>MYSKIKISGTIEVVTGLHIGGGGESSMIGAIDSPVVRDLQTKLPIIPGSSIKGKMRNLLAKHFGLKMKQESHNQDDERVLRLFGSSEKGNIQRARLQISDAFFSEKTKEHFAQNDIAYTETKFENTINRLTAVANPRQIERVTRGSEFDFVFIYNVDEESQVEDDFENIEKAIHLLENDYLGGGGTRGNGRIQFKDTNIETVVGEYDSTNLKIK[4x];> MTIKNYEVVIKTLGPIHIGSGQVMKKQDYIYDFYNSKVYMINGNKLVKFLKRKNLLYTYQNFLRYPPKNPRENGLKDYLDAQNVKQSEWEAFVSYSEKVNQGKKYGNTRPKPLNDLHLMVRDGQNKVYLPGSSIKGAIKTTLVSKYNNEKNKDIYSKIKVSDSKPIDESNLAIYQKIDINKSEKSMPLYRECIDVNTEIKFKLTIEDEIYSINEIEQSIQDFYKNYYDKWLVGFKETKGGRRFALEGGIPDVLNQNILFLGAGTGFVSKTTHYQLKNRKQAKQDSFEILTKKFRGTYGKMKEIPSNVPVALKGTTNQSRHTSYQQGMCKVSFQELNNEVL;> MNKKNILMYGSLLHDIGKIIYRSGDHTFSRGTHSKLGHQFLSQFSEFKDNEVLDNVAYHHYKELAKANLDNDNTAYITYIADNIASGIDRRDIIEEGDEEYEKQLFNFDKYTPLYSVFNIVNSEKLKQTNGKFKFSNESNIEYPKTENIQYSSGNYTTLMKDMSHDLEHKLSIKEGTFPSLLQWTESLWQYVPSSTNKNQLIDISLYDHSRITCAIASCIFDYLNENNIHNYKDELFSKYENTKSFYQKEAFLLLSMDMSGIQDFIYNISGSKALKSLRSRSFYLELMLEVIVDQLLERLELARANLLYTGGGHAYLLVSNTDKVKKKITQFNNELKKWFMSEFTTDLSLSMAFEKCSGDDLMNTSGNYRTIWRNVSSKLSDIKAHKYSAEDILKLNHFHSYGDRECKECLRSDIDINDDGLCSICEGIINISNDLRDKSFFVLSETGKLKMPFNKFISVIDYEEAEMLVQNNNQVRIYSKNKPYIGIGISTNLWMCDYDYASQNQDMREKGIGSYVDREEGVKRLGVVRADIDNLGATFISGIPEKYNSISRTATLSRQLSLFFKYELNHLLENYQITAIYSGGDDLFLIGAWDDIIEASIYINDKFKEFTLDKLTLSAGVGMFSGKYPVSKMAFETGRLEEAAKTGEKNQISLWLQEKVYNWDEFKKNILEEKLLVLQQGFSQTDEHGKAFIYKMLALLRNNEAINIARLAYLLARSKMNEDFTSKIFNWAQNDKDKNQ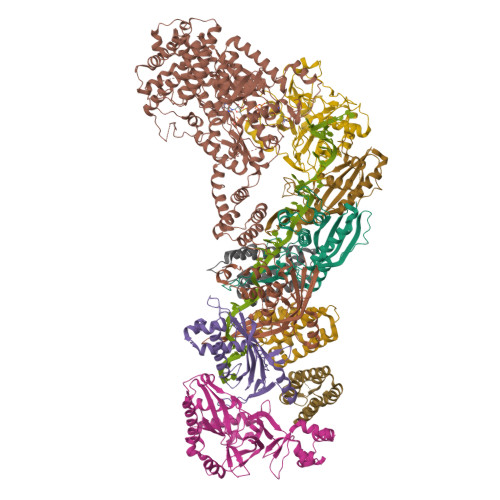LITALEYYIYQIREAD;> MTLATKVFKLSFKTPVHFGKKRLSDGEMTITADTLFSALFIETLQLGKDTDWLLNDLIISDTFPYENELYYLPKPLIKIDSKEEDNHKAFKKLKYVPVHHYNQYLNGELSAEDATDLNDIFNIGYFSLQTKVSLIAQETDSSADSEPYSVGTFTFEPEAGLYFIAKGSEETLDHLNNIMTALQYSGLGGKRNAGYGQFEYEIINNQQLSKLLNQNGKHSILLSTAMAKKEEIESALKEARYILTKRSGFVQSTNYSEMLVKKSDFYSFSSGSVFKNIFNGDIFNVGHNGKHPVYRYAKPLWLEV;>MTFAHEVVKSNVKNVKDRKGKEKQVLFNGLTTSKLRNLMEQVNRLYTIAFNSNEDQLNEEFIDELEYLKIKFYYEAGREKSVDEFLKKTLMFPIIDRVIKKESKKFFLDYCKYFEALVAYAKYYQKED[3x]>MGHHHHHHMSDL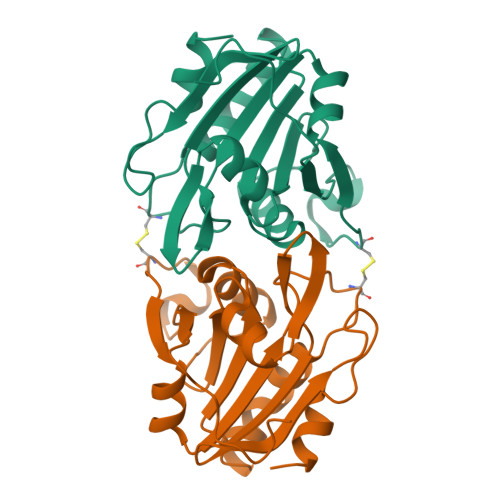VNKKFPAGDYKFQYIAISQSDADSESCKMPQTVEWSKLISENKKVIITGAPAAFSPTCTVSHIPGYINYLDELVKEKEVDQVIVVTVDNPFANQAWAKSLGVKDTTHIKFASDPGCAFTKSIGFELAVGDGVYWSGRWAMVVENGIVTYAAKETNPGTDVTVSSVESVLAHL[4x]Omniligase-1 is a broadly applicable enzyme for peptide bond formation between an activated acyl donor peptide and a non-protected acyl acceptor peptide. The enzyme is derived from an earlier subtilisin variant called peptiligase by several rounds of protein engineering aimed at increasing synthetic yields and substrate range. Mutation A225N in the S1′ pocket and F189W of the S2′ pocket increased the synthesis to hydrolysis (S/H) ratio and overall coupling efficiency, whereas the I107V mutation was added to S4 pocket to increase the reaction rate. The final omniligase variants appeared to have a very broad substrate range, coupling more than 250 peptides in a 400-member library of acyl acceptors, as indicated by a high-throughput FRET assay.

Especially the Ptl variants with mutations M222G/L217F and M222P/L217H proved to have a much broader substrate scope and improved S/H ratio compared to the parent peptiligase. To examine the contribution of individual mutations on S/H ratio and substrate scope in peptide synthesis, we selected peptiligase variant M222P/L217H as a starting enzyme and introduced successive mutations. Inspection of the crystal contacts of Pre-1, Pre-2 and Pre-3 revealed that at position F189 (S2′ pocket) the enzymes in crystal form A as well as in crystal form B have close contact (3.7 Å) with Asn109 of a symmetry-related molecule. A Trp instead of a Phe at position 189 would be too close to this Asn (2.0 Å W189-CD1 to ND1 or OD1 of N109) which cannot adopt a different conformation because of steric hindrance. The different crystal forms show the flexibility of the active site of peptiligases. For instance, His217 is present in two distinct conformations, one pointing into the active site while in the other conformation the sidechain of His217 is facing the solvent. On the other hand, His217 introduced in Oml-1 can rotate away and become exposed to the solvent, enlarging the S1′ cavity and allowing slightly larger P1′ side chains to bind. In conclusion, the L217H + M222P mutations in Oml-1 increase the P1′ tolerance due to an enlarged S1′ cavity that arises when His217 rotates towards the solvent. The effect of all possible mutations on folding stability (ΔΔGfold) was modeled both using the Pre-2 X-ray structure, that carries an Ala at position 225, and the Pre-3 structure, which features Asn225. In an Ala225 template (Pre-2) clearly more strain was visible on both Val68 and Asn225 than when examining the Asn225 template (Pre-3).

> AKCVSYGVSQIKAPALHSQGYTGSNVKVAVIDSGIDSSHPDLNVAGGASFVPSETNPFQDNNSHGTHVAGTVLAVAPSASLYAVKVLGADGSGQYSWIINGIEWAIANNMDVINMSLGGPSGSAALKAAVDKAVASGVVVVAAAGNSGTSGSSSTVSYPAKYPSVIAVGAVDSSNQRAPFSSVGPELDVMAPGVSICSTLPGNKYGAHSGTCPASAHVAGAAALILSKHPNWTNTQVRSSLENTATKLGDSFYYGKGLINVEAAAQHHHHHH>[3x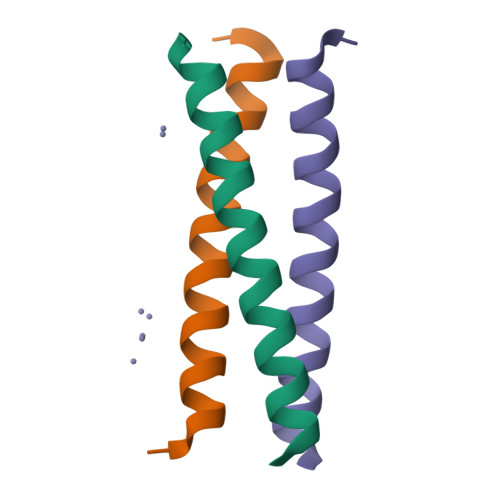]VSRLEEDVRNLNAIVQKLQERLDRLEETVQAK>IINGEDCSPHSQPWQAALVMENELFCSGVLVHPQWVLSAAHCFQNSYTIGLGLHSLEADQEPGSQMVEASLSVRHPEYNRPLLANDLMLIKLDESVSESDTIRSISIASQCPTAGNSCLVSGWGLLANGRMPTVLQCVNVSVVSEEVCSKLYDPLYHPSMFCAGGGQDQKDSCNGDSGGPLICNGYLQGLVSFGKAPCGQVGVPGVYTNLCKFTEWIEKTVQA[7x];>[7x]GSSVVVDTNGQPVSNGADAYYLVPVSHGHAGLALAKIGNEAEPRAVVLDPHHRPGLPVRFESPLRINIIKESYFLNIKFGPSSSDSGVWDVIQQDPIGLAVKVTDTKSLLGPFKV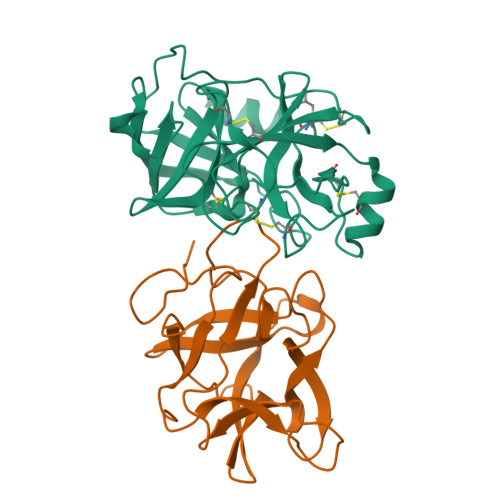EKEGEGYKIVYYPERGQTGLDIGLVHRNDKYYLAVKDGEPCVFKIRKATDE>MQKIGIY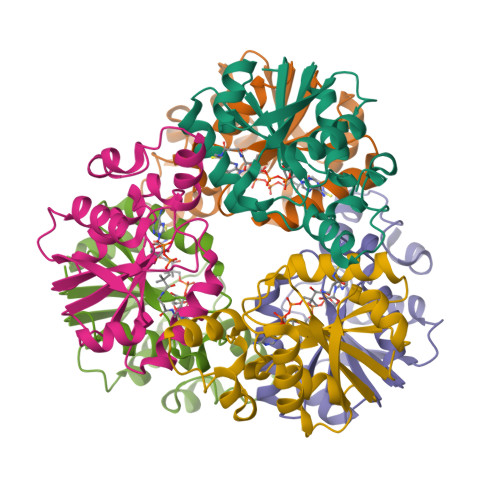AGTFDPVTNGHIDIIHRSSELFEKLIVAVAHSSAKNPMFSLDERLKMIQLATKSFKNVECVAFEGLLANLAKEYHCKVLVRGLRVVSDFEYELQMGYANKSLNHELETLYFMPTLQNAFISSSIVRSIIAHKGDASHLVPKEIYPLIS[6x]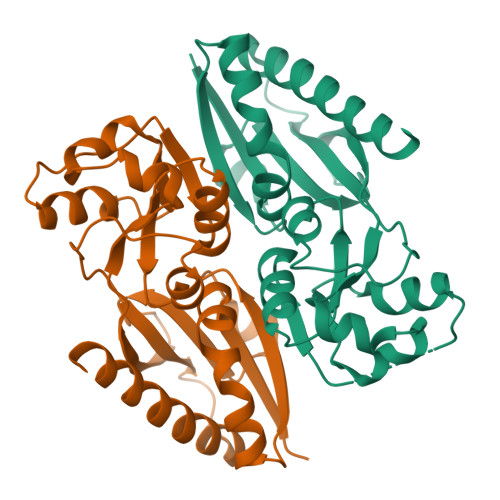>[4x]MLERFEGGHYRDVLTVGAVGTFTVGWLLPRLEDFQARHPFIDLRLSTHNNRVDIAAEGLDYAIRFGGGAWHGTEALALFEAPLTVLCCPEVAAQLHSPADLLQHTLLRSYRADEWPLWFQAAGLPAHAPLTRSIVFDTSLAMLEAARQGVGVALAPAAMFARQLASESIRRPFATEVSTGSYWLTRLQSRGETSAMLAFRGWLLEMAAVEARGRLEHHHHHH> MSHDAQPNEQPNTGIELATGGNGSGSSGGGGRGAGGVGVSTGSFNNQTEFHYLGDGLVQITAHASRLVHLNMPE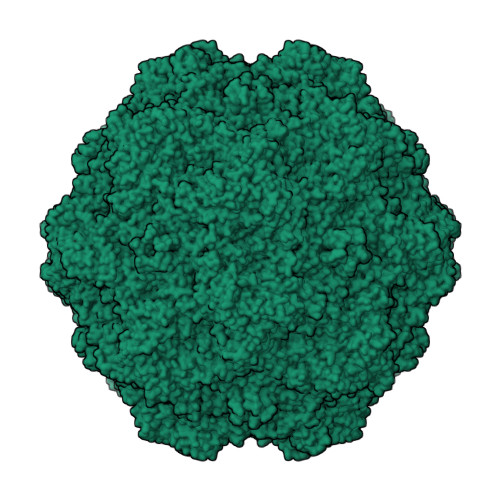HESYRRINVLNSEAGVAGQMVQDDAHSQMVTPWSLVDANAWGVWFNPGDWQLITNNMTELNLVSFEQEIFNVVLKTITESATTPPTKIYNNDLTASLMVALDTNNTLPYTPAAPRSETLGFYPWLPTKPTHYRYYMTCTRNLTPPTHTGQAGTITNTISAPTHSDVMFYTIENAVPIHLLRTGDEFSTGTYYFDTKPLKMTHSWQTNRSLGLPPKLATEPTTEGQQHTGTLKAATDREGIHQTINNSYTEATALRPAQVGYNTPYMNFEYSDGGPFLTPIVPVYDTQYNADEPNGAYRITMGYQHGQITTATELGRYTLNPISKGGRAPNQEFNQSSPLQMENTLNGTLLPTDPIGGKTDIHFTNTLNTYGPLTALNNTPPIYPNGQIWDKELDADLKPRLHVTAPFVCKNNPPGQLFVKIAPNLTDDFNADSPQQPRIITYSNFWWKGTLTFTARMRSSNMWNPIHQHTTTNDNIVNYMPSNIGGMRLYPEIPQLIPRKLY>MAKLTSAVPVLTARDVAGAVEFWTDRLGFSRDFVEDDFAGVVRDDVTLFISAVQDQVVPDNTLAWVWVRGLDELYAEWSEVVSTNFRDASGPAMTEIGEQPWGREFALRDPAGNCV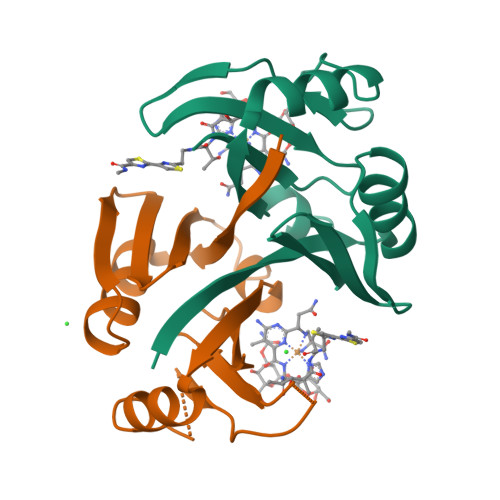HFVAEEQD[2x]>MPDKAEYLLAINCGSSSIKGKLFAIPSFELLANLAVTNISSSDERVKIKTTWEEGKGKDSEEEADYGDKIRYASLVPILLDHLTNSTHVKKEEIKYVCHRVVHGGMHDKGIRVVKGHEEGLMEMDKLSEFAPLHNHRAVLAVKSCIDALPHHTSLLLFDTIFHRTIAPEVYTYALPPPDTELTMPLRKYGFHGLSYASIVQSLAEHLKKPSDQINVVVAHLGSGSSSCCIKNGKSIDTSMGLTPLEGLLGGTRSGTIDPTAIFHHTEDAASDANVGDFTVSKAEIILNKNSGFKALAGTTNFGHIIQNLDPSKCSEEDHEKAKLTYAVFLDRLLNFVAQYLFKLLSEVPIESIDGLVFSGGIGEKGAELRRDVLKKLAWLGAEVDEEANNSNSGGAVKCITKEGSKLKGWVVETDEEGWMARM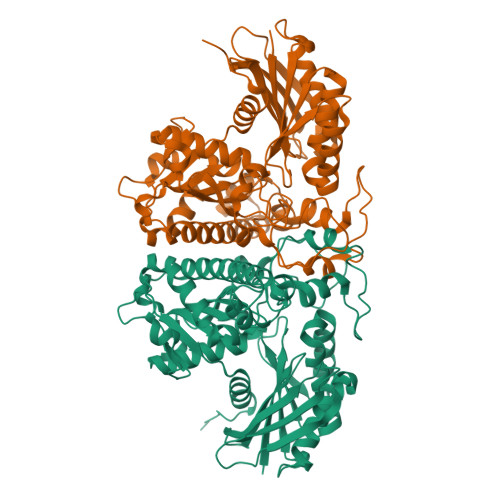AKEEFGFLEHHHHHH[2x]>[2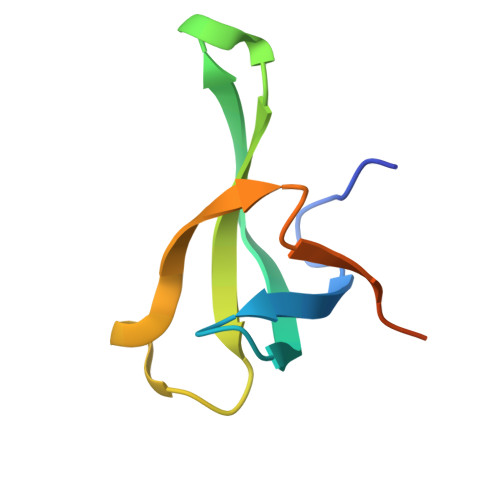x]MVMFEVRQKVYATLHETFHAAIIQEVAHDAHTGQLLYYVHYVEQDSRMDRWLPGSALRERRQGLEHHHHHH>[3x]GSSGSSGMQIGKIIKVSGPLVMAENMSEASIQDMCLVGDLGVIGEIIEMRQDVASIQVYEETSGIGPGEPVRSTGEALSVELGPGIISQMFDGIQRPLDTFMEVTQSNFLGRGVQLPALDHEKQWWFEATIEEGTEVSAGDIIGYVDETKIIQHKIMVPNGIKGTVQKIESGSFTIDDPICVIETEQGLKELTMMQKWPVRRGRPIKQKLNPDVPMITGQRVIDTFFPVTKGGAAAVPGPFGAGKTVVQHQIAKWSDVDLVVYVGCGERGNEMTDVVNEFPELIDPNTGESLMERTVLIANTSNMPVAAREASIYTGITIAEYFRDMGYDVAIMADSTSRWAEALREMSGRLEEMPGDEGYPAYLGSRLAEYYERSGRVIALGSDQREGSITAISAVSPSGGDISEPVTQNTLRVVKVFWGLDSSLAQKRHFPSINWIQSYSLYSTEVGRYMDQILQQDWSDMVTEGMRILQEEEQLNEIVRLVGIDSLSDNDRLTLEVAKSIREDYLQQNAFDDVDTFTSREKQFNMLKVILTFGKEARKALSLGAYFNEIMEGTVAVRERISRSKYIPEEELAKISSINEEIKETIQLIVSEGGMTDD;>[3x]GSSGSSGMIKEYRTIKEVVGPLMAVEKVSGVKYEELIEVRMQNGEIRRGQVLEVQEDKAMVQIFEGTSGINLKNSSVRFLGHPLQLGVSEDMIGRVFDGLGRPKDNGPEILPEKYLDINGEVINPIARDYPDEFIQTGISAIDHLNTLVRGQKLPVFSGSGLPHKELAAQIARQATVLDSSDDFAVVFAAIGITFEEAEFFMEDFRQTGAIDRSVMFMNLANDPAIERIATPRMALTAAEYLAYEKGMHVLVIMTDMTNYAEALREISAARREVPGRRGYPGYLYTNLATLFERAGRIRGLKGSVTQIPILTMPEDDKTHPIPDLTGYITEGQIILTRELYKSGIQPPIDVLPSLSRLKDKGTGAGKTREDHAATMNQLF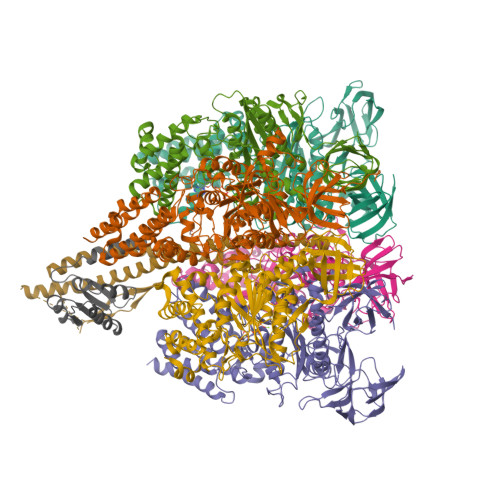AAYAQGKQAKELAVVLGESALSDIDKIYAKFAERFENEYVNQGFYTNRTITETLDLGWELLAMLPRTELKRIKDDLLDKYLPEGK;> GSSGSSGMRLNVNPTRMELTRLKKQLTTATRGHKLLKDKQDELMRQFILLIRKNNELRQAIEKETQTAMKDFVLAKSTVEEAFIDELLALPAENVSISVVEKNIMSVKVPLMNFQYDETLNETPLEYGYLHSNAELDRSIDGFTQLLPKLLKLAEVEKTCQLMAEEIEKTRRRVNALEYMTIPQLEETIYYIKMKLEENERAEVTRLIKVKNMGTEE;> MTYKIGVVGDKDSVSPFRLFGFDVQHGTTKTEIRKTIDEMAKNEYGVIYITEQCANLVPETIERYKGQLTPAIILIPSHQGTLGIGLEEIQNSVEKAVGQNILSGPSSGENLYFQ> MALLMEGGDPMSVDGSSTMPAHMRVMPDMGITGAPMTLDDVDLFGDAVMNNALDALPPAPGHPPPSRALQRRIAELRARGCCQGIAWSRQGTIASISADGMSIELRFLRTNPENGDWELT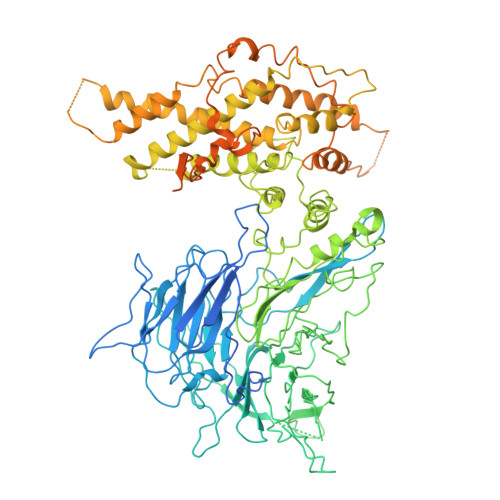DAALSLSVALVPASSPSATSSSGSGTSNTTVISAGAPFVHLAWAPSVHTSSFELAAIDAPGRITIFLFTQNINKPYLSRKWDTDPVDDLHAVVGCYWLPLPFNVSYVANWVQTDYRYEPILSPAWGPIHPNHTKSALVCVTTNGLLKMLFPQNNNRIEETSIELESVTASDDLITHAAIGADRNTLLIALAMGSKQLRVVRVGIQWWLPQVDKQQMPPSVPLRPSLRESRVAVTTLLDPEQQQSDGDAPIAQLTHLEILPSPLGETPQTVLPPVILAVRSYLPQEGSLYAAHQEPFTVIDRWELFTDQPKAFHPAFEQLGAKNSASSQPSAMQTLRKLDPVVIPGKVVVTVNTLQFGRVVCFGFSDGTLQYRDRFTMNEVYTEQATTNITSPLQVGFQWETEGPCLQMAFAPTNCSFVQVSEDGSVKWVKLRYPVDDPNMTLQGPKLKAVAASLAVASVGANIAGPNIHNHCDDVMAIARPLAKKFKDFPTAWVREFVTMFKITVDYSEEAHHDQLMRNSLLQFCLSILNHFGFNGDFQPRTFSGKFANLALAVRNIVVLITIASNAPNTIKEKLSPLDEPEVVDALASCAKWGFDLLAWLTDRLLALSTDQTIKAMLADQKRFPDLARYLHSKNDVSLHLLLCSSTRGLLSAVCRRLQVVESLAHRATVYYESRYAVDPAAAAQKTLPPLYHAYVKMQRVVTASLVKASDFDKLLTALSRDIQTAYIQTFSGVATQIRQHASGSGGQPLTEQQQQQCNEQFIKKAQSHVELDMLLGQNPPPGFREVLACFFGNIFPAFRATVDPRSVFFADWSLLEEIVAEDERTLKRRREGGGRYVDVFKRVELCGRGQVLPRGRIVASVKTERAEAVPMVPSQSQSSHQAASQAQGQQSQQQQGATPAPNATPSVPISQLNPPTGPTQPPNSSGNTANANPNTGTNANTLGGSVPGLQGFVPVTANLAVNASQWRRCVRCAAVMEDVWGQRPGFTFVLTQQRRCACGGGWGLVPRGD> MTLSIPPSIQCQTEAACRLITRVTGDTLRAIHLYGSAVAGGLKPNSDIDLLVTICQPLTEAQRATLMQELLALSSPPGASAEKRALEVTVVLYSQLVPWCFPPSREMQFGEWLREDICQGIYEPAQQDWDMVLLITQILETSIPLKGERAERLFTPAPAAQLLKALRYPLDLWQSTADVQGDEYHIVLTLARIWYTLSTGRFTSKDAAADWLLPQLPEDYAATLRAA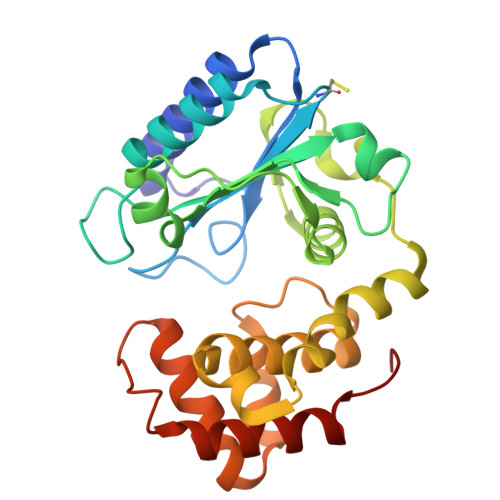QREYLGLEQQDWHILLPAVVRFVDFAKAHIPTQFTKG> MPNGQTKPL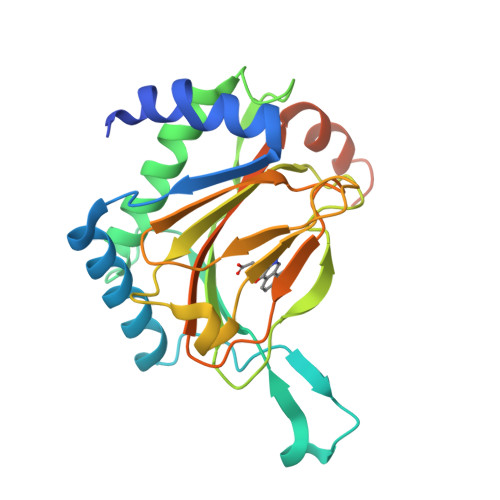PALKLALEYIVPCMNKHGICVVDDFLGKETGQQIGDEVRALHDTGKFTDGQLVSQKSDSSKDIRGDKITWIEGKEPGCETIGLLMSSMDDLIRHCNGKLGSYKINGRTKAMVACYPGNGTGYVRHVDNPNGDGRCVTCIYYLNKDWDAKVSGGILRIFPEGKAQFADIEPKFDRLLFFWSDRRNPHEVQPAYATRYAITVWYFDADERARAKVKYLTGEKGVRVELNKPHHHHHH>[2x]TTVGFSQVGSESGWRTSFSEAVKAEAKQRGIDLKFADAQQKQENQIKAVRSFIAQGVDAIIIAPVVETGWKPVLKEAKRAKIPVVIVDRNIKVDDDSLFLTRIASDFSEEGRKIGQWLMDKTQGNCDIAELQGTVGATAAIDRAAGFNQVIANYPNAKIVRSQTGEFTRAKGKEVMEGFLKAQNGQPLCAVWSHNDEMALGAVQAIKEAGLKPGKDILIVSVDGVPDYFKAMADGDVNA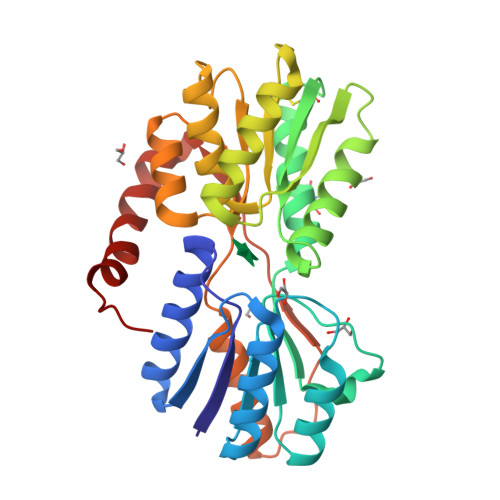TVELSPYLGGPAFDAIDAYLKGNKDQAKLISTTGDVFTQETAAAEYEKRRQQAAALEHHHHHH bis(4-hydroxyphenyl)methanone | C13 H10 O3 | 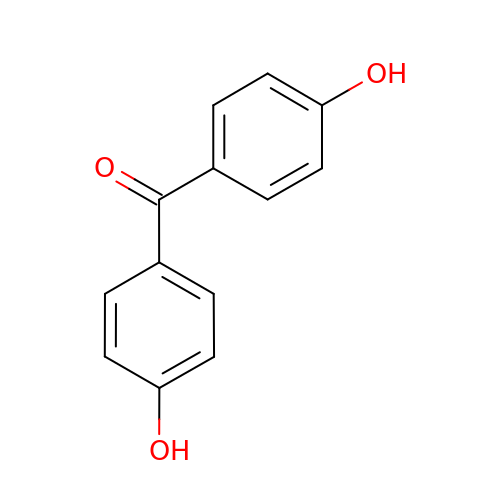RXNYJUSEXLAVNQ-UHFFFAOYSA-N> MENTSSMKEMATLLTSLGVIQSAQEFESSRDASYVFARRALKSANYAEMTFNVCGLILSAEKSS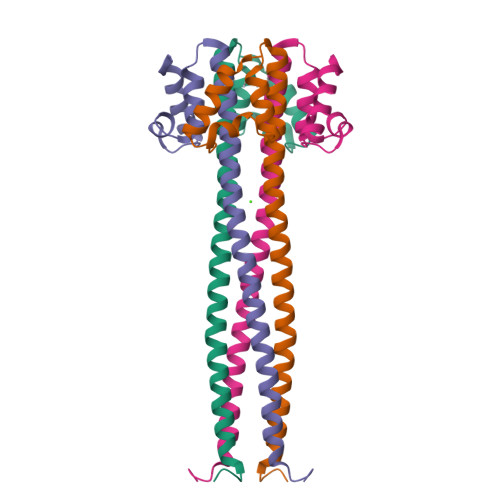ARKVDENKQLLKQIQESVESFRDIYKRFSEYQKEQNSLLMSNLSTLHIITD> HMASMTGGQQMGRRRSEKSRVAIVEATRALLLERGFDGLSIEAVAAKAGVGKQTIYRWWPSRHALVADVLLEDADKILARMPKTDDVTADLASWAGTLAAALTTRRGHAMLKTLMAASLEHEDTAARLREGFSRPLIESVRDRLRDEDIDADHAQAAADALLGAVVNAVLSEGR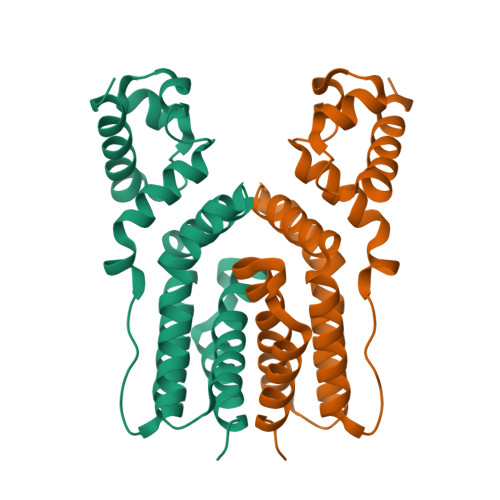SYSRQRAETSARIIVAGLRP>MSAIRDVMTKFAEQTTMHGVPKVINAKSSMGRLFWSLVCLAAGAMFCLQMSEVLQRYFSYPKKVTVEVVPTPVPFPSISICNMRNLDVHILNTLNRMFIEDDRPFSNINKSEHEFIRAYMKKVAKYAPLFWNYQDEYPEVFQEIFSRTTFSANIDPEVIALAAVQLEGFVVNCHYAGHRCNKTRDFYRFFDPYYFNCFTYKAHEPTDIEDNLSEGIENGWSSILLSGSGMLDKNDEIRMLPGLHEWRSAVSASEGVRVVIHPPSTTPYPFTEGYDVPPGFSASFGIHPRRNIRIGPPHGNCSDKNPFGDGTERYRLMACQKMCMQHYIVETCGCADVGLPKLPLQANISWCRDDDNFPDECMFTASEECLQLLMQLHNRIKCARSIKSKITKNTTAMEACNCFPPCDEVSYDVSYSLSKWPSAGYEGDAAYFDVFGIEKFNERFNKTGTQGKYELFTKYFNVSNREESMKDFARLNVYIADSNVVKTQESEDYTRNQLVSDIGGQLGLWVGISLITLAEVLELIIDLFRLFSKHTYRSVPVIRQSIKYKDKRNGAEMNYDTRYSQSNGGPHARYLHHGHSIPKHPPELPDTSLALEVLFQ[3x];>[3x]FMRFX

Here we dissected the structural basis for neuropeptide-gated activity of a neuropeptide-gated DEG/ENaC, FMRFamide-gated sodium channel 1 (FaNaC1) from the annelid worm Malacoceros fuliginosus, using cryo-electron microscopy. We solved high-resolution structures of FaNaC1 alone, with full agonist FMRFa, with partial agonist ASSFVRIa, and with both FMRFa and pore-blocker diminazene, identifying the ligand-binding site and elucidating the conformational changes induced by ligand binding. Each subunit comprises a minimal N terminus and a nonresolved 63-amino acid C terminus facing the intracellular side, two transmembrane segments (TM1 and TM2), and a large extracellular domain. The FaNaC1 structures presented here capture a ligand-free resting state, two ligand-bound desensitized states and a ligand-bound dilated channel state.

In solving the FaNaC1/FMRFa/diminazene structure, several 3D classes emerged during our image analysis, with two predominating: a closed-channel class similar to the FaNaC1/FMRFa structure; and a class that differed from the others with dilated mid- to upper pore, and some probably nonprotein density in the channel pore. We focused on this second 3D class, resolving the structure to 3 Å resolution. We easily modeled TM2 helices into the cryo-EM density and observed an ~1 Å increase in the pore radius relative to our other structures. Although the resolved density in the pore was too small to accommodate a full diminazine molecule, no such density or dilated conformation was observed in the diminazine-free FMRFa-bound dataset, suggesting that diminazene binds and affects FaNaC1 pore conformation. Given the drug’s effect on pore radius and its voltage-dependent block of currents, we hypothesized that this nonprotein density derives from partially unresolved or low occupancy diminazene molecules. Thus, we interpret our FaNaC1/FMRFa/diminazene structure as an FMRFa-gated, diminazene-blocked, open-channel conformation. In its binding pocket, FMRFa draws the C-terminal end of α2 and α3a (distal finger domain) 3–5 Å upward and inward in the direction of α6 of the adjacent subunit, whereas the N-terminal end of α2, α3b/α3c and all of α6 (knuckle) are relatively static. The net result of peripheral movement on internal stasis is that the extracellular domain of a single subunit rolls anticlockwise (viewed from above) and upward (viewed from the side). Extracellular domain rolling pulls the β-turn at the proximal-thumb/wrist domain outward, which couples to upper-channel expansion via β-turn H297 interactions with TM1 Y59 and TM2a E490. Lower-pore dilation is similar in both FaNaC1/FMRFa/diminazene and FaNaC1/FMRFa structures, in contrast to upper-pore dilation, which is present in the FaNaC1/FMRFa/diminazene structure but collapsed in the desensitized FaNaC1/FMRFa structure.In this context, we recently reported the characterization of a novel xyloglucan utilization locus (XyGUL) that confers Bacteroides ovatus, and species harbouring syntenic XyGULs, with the ability to utilize this abundant vegetable polysaccharide across sampled human populations. Here, we present the three-dimensional structures of BoGH31, BoGH43A, BoGH43B and BoGH3B, expanding our knowledge of the structural determinants required for xyloglucan degradation. Our analyses highlight key adaptations in these enzymes that confer their specificity for xyloglucan oligosaccharides, while also providing a rationale for the maintenance of two divergent genes coding for GH3 enzymes, and similarly two divergent genes for GH43 family members, within the same PUL. While we were unable to determine a structure for BoGH3A, our structural and sequence analysis of BoGH3B has also allowed us to highlight further potential differences between these two enzymes encoded by the operon. Together with existing biochemical data, our analyses of the three-dimensional structures, and various enzyme-inhibitor complexes, of BoGH31, BoGH43A, BoGH43B and BoGH3B provide molecular-level insight into the stepwise breakdown of xyloglucan by the BoXyGUL.

Despite significant functional overlap with BoGH43A, BoGH43B, the second α-l-arabinofuranosidase present in the BoXyGUL, shares just 41% sequence identity with BoGH43A and appears to be significantly less active on the substrates tested. Crystals of BoGH43B were obtained by hanging drop vapour diffusion using 0.2 M sodium acetate pH 5, 20–30% PEG-3350 as mother liquor and they were used for subsequent structure determination. Remarkably, given their apparent differences at the amino acid level, the structure of BoGH43B appears extremely similar to that of BoGH43A, which can be superimposed onto BoGH43B, using GESAMT, with an RMSD of 1.24 Å over 482 amino acid residues. Comparison of tertiary folds reveals few significant differences between the two paralogues, with the most obvious being the presence of a metal binding site, occupied by calcium, towards the C-terminus of BoGH43B. Such an equivalent site appears entirely absent within BoGH43A. However, the Ca2+-binding site in BoGH43B is located in the C-terminal β-sandwich domain, on the opposite side of the molecule from the active site, and similar sites in other family members have not been implicated in catalysis to date. Superposition of apo-BoGH43B with AraDNJ-BoGH43A reveals that the three residues implicated in catalysis (Asp38, Asp148 and Glu198 in BoGH43B) are absolutely conserved. The only difference in the BoGH43B −1 sub-site is the replacement of Phe93 (in BoGH43A) with a tyrosine residue in BoGH43B. AraLOG stacks against Tyr187 in BoGH43A, which is replaced by Ser196 in BoGH43B.

>[2x]MQKTFRNPIITGMNPDPSICRVGDDFYLVTSTFEYFPGLPVYHSKDLVHWKLIGHALSRPENNPLMGCNASTGGQYAPTLRYHDGTFYVIGTNYGGKGSQGVFYVTAKNPAGPWSDPVWVGNWYVDPSIEFIDGKMYFLSPDNQGSFLLGVMDPETGTFVEALRKVASGLGGSSPEGPHFYKIGDYYYIMSAEGGTGYEHREVIQRSKSPWGPYEPSPVNPVLSNMNCPDHPFQAIGHADLVQLKDGSWWAVCLGIRPVNGKYQHLGRETFLAPVTWDADGWPKVGKDGVVQETYLFPNLPSHVWMEQPVRDDFDQETLGLDWTFIRNPAHSFWSLTEKPGSLRLKGTAINFTTNDSPSFIGRRQAAFNLTASAKVNFIPKVENEEAGLVVRADDKNHYDLLITERNGQRVAMIRKTLKDKVVDTTCKELPATGEVILSITATETTYTFEIKAAHVSAILGTASTRDVSNEVVGGFTGVFIGMYASGNGQANTNPADFDWFDFRCLDLEHHHHHH>[4x]GSHMENSWTISKEYHIDEEVGFALPNPQENLPDFYNDWMFIAKHLPDLIESGQLRERVEKLNMLSIDHLTDHKSQRLARLVLGCITMAYVWGKGHGDVRKVLPRNIAVPYCQLSKKLELPPILVYADCVLANWKKKDPNKPLTYENMDVLFSFRDGDCSKGFFLVSLLVEIAAASAIKVIPTVFKAMQMQERDTLLKALLEIASCLEKALQV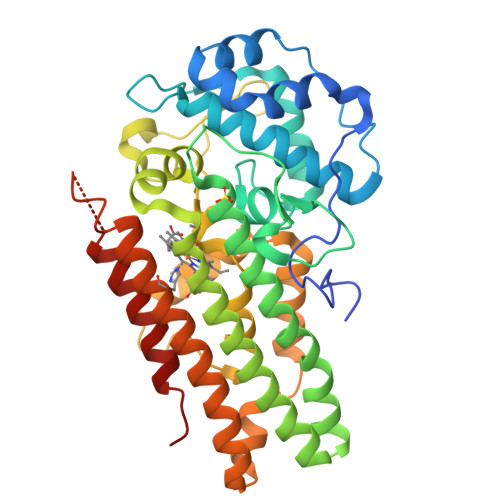FHQIHDHVNPKAFFSVLRIYLSGWKGNPQLSDGLVYEGFWEDPKEFAGGSAGQSSVFQCFDVLLGIQQTAGGGHAAQFLQDMRRYMPPAHRNFLCSLESNPSVREFVLSKGDAGLREAYDACVKALVSLRSYHLQIVTKYILIPASQQPKENKTSEDPSKLEAKGTGGTDLMNFLKTVRSTTEKSLLKEG>AT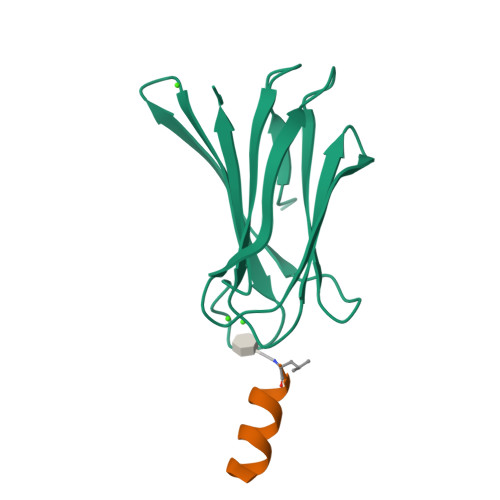QGVFTLPANTRFGVTAFANSSGTQTVNVLVNNETAATFSGQSTNNAVIGTQVLNSGSSGKVQVQVSVNGRPSDLVSAQVILTNELNFALVGSEDGTDNDYNDAVVVINWPLG[4x];>LLKALKKLAKKY[4x]>MQDNSRYTHFLTQHYDAKPQGRDDRYCESIMRRRGLTSPCKDINTFIHGNKRSIKAICENKNGNPHRENLRISKSSFPVTTCKLHGGSPWPPCQYRATAGFRNVVVACENGLPVHLDQSIFRRP[4x]

Angiogenin (ANG), a 14-kDa basic protein is an angiogenic ribonuclease and member of the bovine pancreatic ribonuclease (RNase A) family (also known as RNase 5). Like RNase A, ANG cleaves preferentially on the 3′ side of pyrimidines and follows a transphosphorylation/hydrolysis mechanism. In addition, the crystal structure of human ANG has revealed that it has an RNase A fold and the catalytic triad (residues H13, K40 and H114) is conserved. The enzymatic activity of ANG is several orders of magnitude lower than that of RNase A towards conventional RNase substrates, but essential for its angiogenic effect.

The residue Q77 forms part of the β4 strand in the ANG wild-type structure. So far there is no assigned role for this residue. However, in the Q77P PD variant structure (which contains 4 molecules in the asymmetric unit with clear electron density for the proline ring, which is less accessible to solvent) the hydrogen-bond (2.9 Å) observed between Q77 and R21 (part of helix α2) is lost thus creating a hydrophobic environment. However, in the variant structure, residue P77 also retains van der Waals contacts with residues I46 and F100 that are in close proximity to the substrate binding site. However, these structural changes might contribute for the loss (~40%) of enzyme activity.> LVVPNINSSNPTTSNSAPALDAAETGHTSSVQPEDVIETRYVQTSQTRDEMSLESFLGRSGCIHESKLEVTLANYNKENFTVWAINLQEMAQIRRKFELFTYTRFDSEITLVPC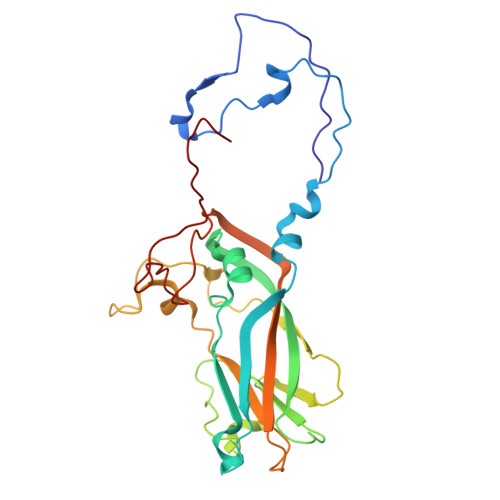ISALSQDIGHITMQYMYVPPGAPVPNSRDDYAWQSGTNASVFWQHGQAYPRFSLPFLSVASAYYMFYDGYDEQDQNYGTANTNNMGSLCSRIVTEKHIHKVHIMTRIYHKAKHVKAWCPRPPRALEYTRAHRTNFKIEDRSIQTAIVTRPIITTA>ALWQFNGMIKCKIPSSEPLLDFNNYGCYCGLGGSGTPVDDLDRCCQTHDNCYMQAMKLDSCKVLVDNPYTNNYSYSCSNNEITCSSENNACEAFICNC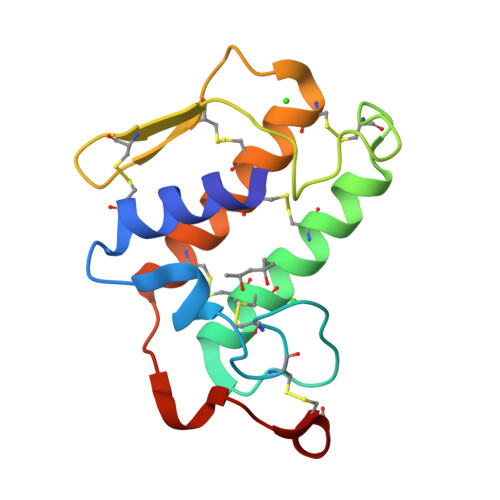DRNAAICFSKVPYNKEHKNLDMMNC[2x]> KPVIKMYQIGDKPDNLDELLANANKIIEEKVGAKLDIQYLGWGDYGKKMSVITSSGENYDIAFADNYIVNAQKGAYADLTELYKKEGKDLYKALDPAYIKGNTVNGKIYAVPVAANVASSQNFAFNGTLLAKYGIDISGVTSYETLEPVLKQIKEKAPDVVPFAIGKVFIPSDNFDYPVANGLPFVIDLEGDTTKVVNRYEVPRFKEHLKTLHKFYEAGYIPKDVATSDTSFDLQQDTWFVREETVGPADYGNSLLSRVANKDIQIKPITNFIKKNQTTQVANFVISNNSKNKEKSMEILNLLNTNPELLNGLVYGPEGKNWEKIEGKENRVRVLDGYKGNTHMGGWNTGNNWILYINENVTDQQIENSKKELAEAKESPALGFIFNTDNVKSEISAIANTMQQFDTAINTGTVDPDKAIPELMEKLKSEGAYEKVLNEMQKQYDEFLKNKK

The genome of S. pneumoniae contains genes that encode a suite of proteins that are biochemically capable of performing the various concerted steps needed to completely depolymerize and transport all classes of N-glycans found on host glycoconjugates. Here we characterize SpGH92 (TIGR4 locus tag SP_2145) as an α-mannosidase that trims the terminal α-(1,2)-linked mannose residues on high-mannose glycans to generate a substrate for EndoD. We also identify a solute binding protein (SBP; NgtS) from an ABC transporter (ABCNG) that binds soluble N-glycans and, through X-ray crystallography, reveal the molecular basis of its interaction with these branched glycans. The identification of an ABC transporter that possesses an SBP, NgtS, that is specific to the recognition of N-glycan fragments suggests that this is likely the convergence point of the complex and high mannose N-glycan processing sides of the N-glycan degradation pathway, with this transporter functioning to import soluble N-glycan fragments into the bacterium.

We tackled this hypothesis through a functional and structural analysis of SP_0092, the putative cell-surface attached SBP of the ABC transporter, which we refer to as NgtS (N-glycan transport SBP). NgtS in its unbound form formed crystals in the space group P21 that were sufficiently robust to withstand soaking in high concentrations of sodium iodide to generate a halide derivative. The structure of NgtS is similar to that of other SBPs and comprises two α/β domains separated by a hinge region. Each α/β domain consists of a central β-sheet of three β-strands flanked by α-helices, with the N-terminal domain possessing an additional solvent-exposed two-stranded β-sheet. As with other SBPs, the ligand-binding site was found at the interface of the two domains comprising NgtS and ligand recognition involves a transition from the open, unbound form to a ligand-stabilized closed form. Despite these two complexes being obtained with different ligands and in different spacegroups, the overall conformations of NgtS were very similar (rmsd of 1.0 Å over 427 matched Cα positions); both complexes were in a “closed” conformation relative to the “open” conformation obtained in the absence of ligand.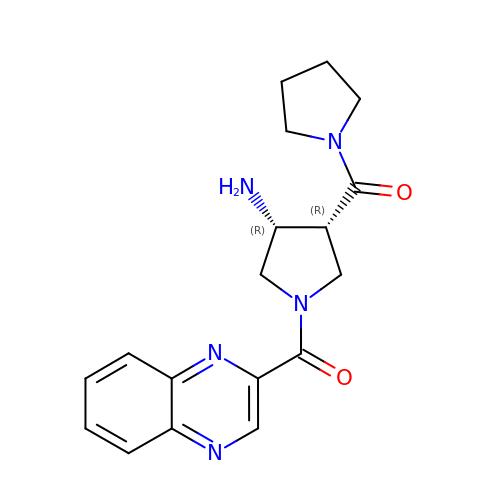(3R,4R)-4-(pyrrolidin-1-ylcarbonyl)-1-(quinoxalin-2-ylcarbonyl)pyrrolidin-3-amine | C18 H21 N5 O2 | XDSKICAQKGYYJF-OLZOCXBDSA-N> ASNLKIVRMDRTAGCVTGGEEIYLLCDKVQKDDIQIRFYEEEENGGVWEGFGDFSPTDVHRQFAIVFKTPKYKDVNITKPASVFVQLRRKSDLETSEPKPFLYYPEIKDKEEVQRKRQKL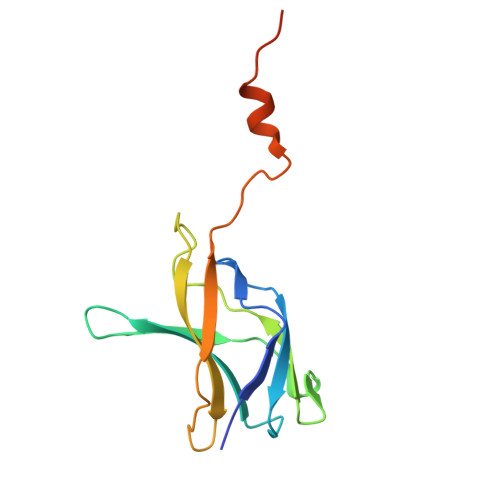MPNFSDSFGGGS>[2x]MSIVNESGSQPVVSRDETLSQIERTSFHISSGKDISLEEIARAARDHQPVTLHDEVVNRVTRSRSILESMVSDERVIYGVNTSMGGFVNYIVP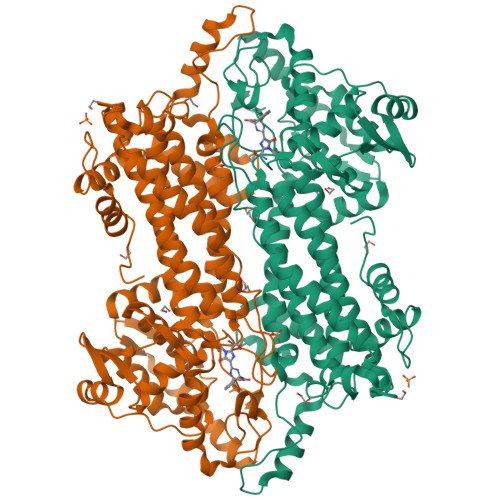IAKASELQNNLINAVATNVGKYFDDTTVRATMLARIVSLSRGNSAISIVNFKKLIEIYNQGIVPCIPEKGSLGXDLGPLAAIALVCTGQWKARYQGEQMSGAMALEKAGISPMELSFKEGLALINGTSAMVGLGVLLYDEVKRLFDTYLTVTSLSIEGLHGKTKPFEPAVHRMKPHQGQLEVATTIWETLADSSLAVNEHEVEKLIAEEMDGLVKASNHQIEDAYSIRCTPQILGPVADTLKNIKQTLTNELNSSNDNPLIDQTTEEVFHNGHFHGQYVSMAMDHLNIALVTMMNLANRRIDRFMDKSNSNGLPPFLCAENAGLRLGLMGGQFMTASITAESRASCMPMSIQSLSTTGDFQDIVSFGLVAARRVREQLKNLKYVFSFELLCACQAVDIRGTAGLSKRTRALYDKTRTLVPYLEEDKTISDYIESIAQTVLTKNSDILEHHHHHH> GSPPKGPELSLASIHVPLESIKPSSALPVTAYDKNGFRILFHFAKECPPGRPDVLVVVVSMLNMAPLPVKSIVLQAAAPKSMKVKLQPPSGTELSPFSPI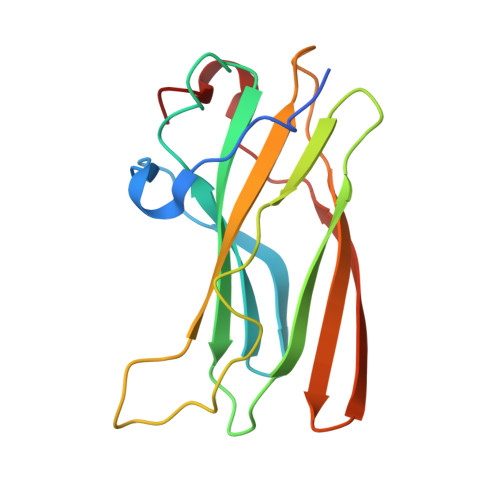QPPAAITQVMLLANPLKEKVRLRYKLTFALGEQLSTEVGEVDQFPPVEQWGNL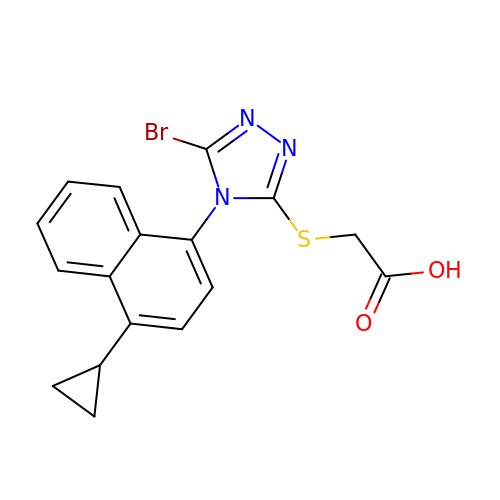lesinurad | C17 H14 Br N3 O2 S | FGQFOYHRJSUHMR-UHFFFAOYSA-N> GFCCPSHWSSYDRYCYKVFKQEMTWADAEKFCTQQHTGSHLVSFHSTEEVDFVVKMTHQSLKSTFFWIGANNIWNKCNWQWSDGTKPEYKEWHEEFECLISRTFDNQWLSA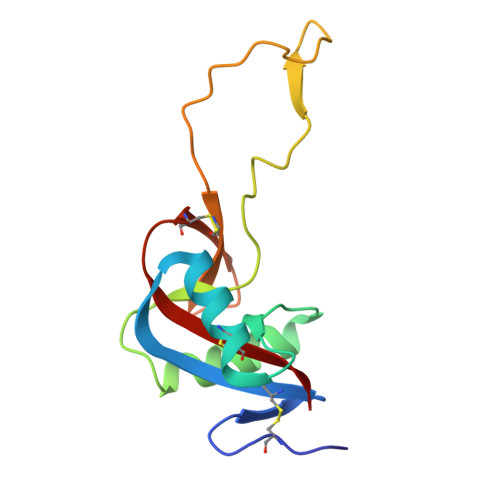PCSDTYSFVCKFEA>GHMYEVDHADVYDLFYLGRGKDYAAEASDIADLVRSRTPEASSLLDVACGTGTHLEHFTKEFGDTAGLELSEDMLTHARKRLPDATLHQGDMRDFRLGRKFSAVVSMFSSVGYLKTTEELGAAVASFAEHLEP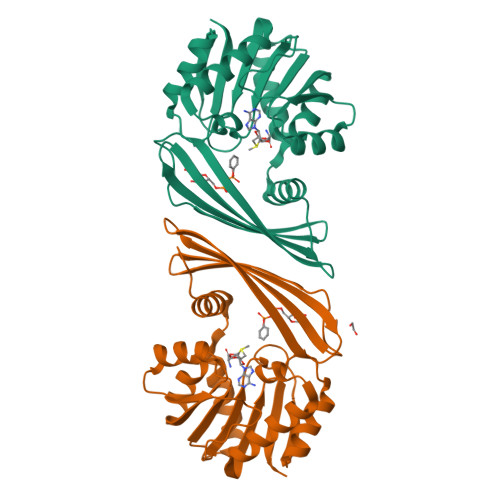GGVVVVEPWWFPETFADGWVSADVVRRDGRTVARVSHSVREGNATRMEVHFTVADPGKGVRHFSDVHLITLFHQAEYEAAFTAAGLRVEYLEGGPSGRGLFVGVPA[2x]(1~{R},3~{S},5~{Z})-4-methylidene-5-[(~{E})-3-[3-(6-methyl-6-oxidanyl-heptyl)phenyl]hex-2-enylidene]cyclohexane-1,3-diol 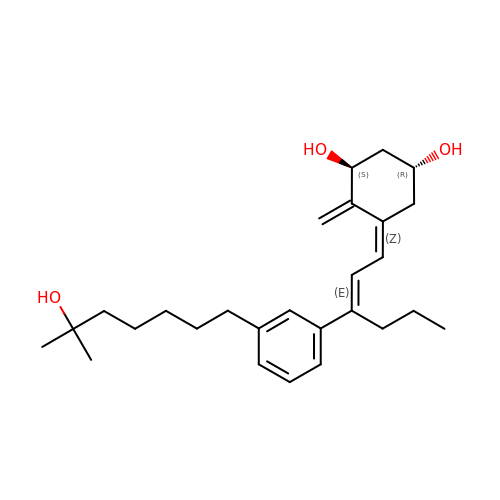| C27 H40 O3 | BFVRWKHYESORKD-HAQBNOSQSA-N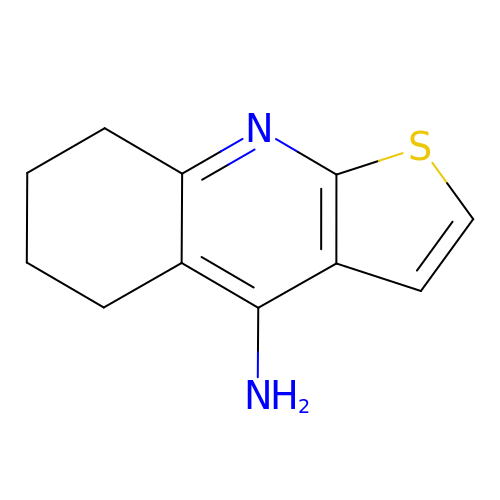5,6,7,8-tetrahydrothieno[2,3-b]quinolin-4-amine | C11 H12 N2 S | PMWMMNQYOBSEDT-UHFFFAOYSA-N>MSGADRSPNAGAAPDSAPGQAAVASAYQRFEPRAYLRNNYAPPRGDLCNPNGVGPWALRCLAQTFATGEVSGRTLIDIGSGPTVYQLLSACSHFEDITMTDFLEVNRQELGRWLQEEPGAFNWSMYSQHACLIEGKGECWQDKERQ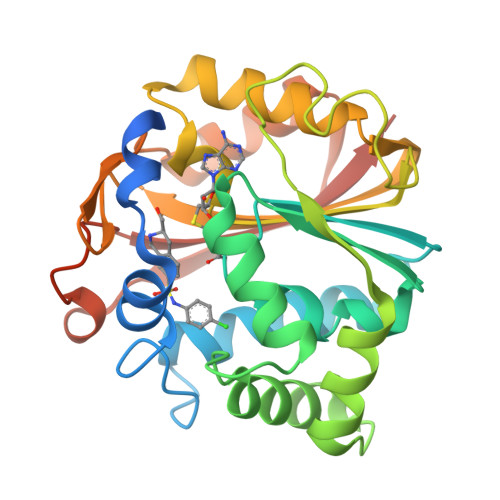LRARVKRVLPIDVHQPQPLGAGSPAPLPADALVSAFCLEAVSPDLASFQRALDHITTLLRPGGHLLLIGALEESWYLAGEARLTVVPVSEEEVREALVRSGYKVRDLRTYIMPAHLQTGVDDVKGVFFAWAQKVGLEHHHHHH[2x]>[2x]GSKPFTVPILTVEEMTNSRFPIPLEKLFTGPSGAFVVQPQNGRCTTDGVLLGTTQLSPVNICTFRGDVTHIAGSRNYTMNLASLNWNNYDPTEEIPAPLGTPDFVGKIQGLLTQTTKGDGSTRGHKATVYTGSAPFTPKLGSVQFSTDTENDFETHQNTKFTPVGVIQDGSTTHRNEPQQWVLPSYSGRNVHNVHLAPAVAPTFPGEQLLFFRSTMPGCSGYPNMDLDCLLPQEWVQHFYQEAAPAQSDV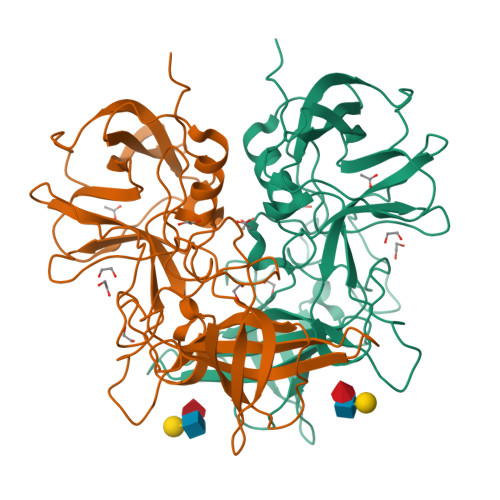ALLRFVNPDTGRVLFECKLHKSGYVTVAHTGQHDLVIPPNGYFRFDSWVNQFYTLAPM> PNFSGNWKIIRSENFEELLKVLGVNVMLRKIAVAAASKPAVEIKQEGDTFYIKVSTTVRTTEINFKVGEEFEEQTVDGRPCKSLVKWE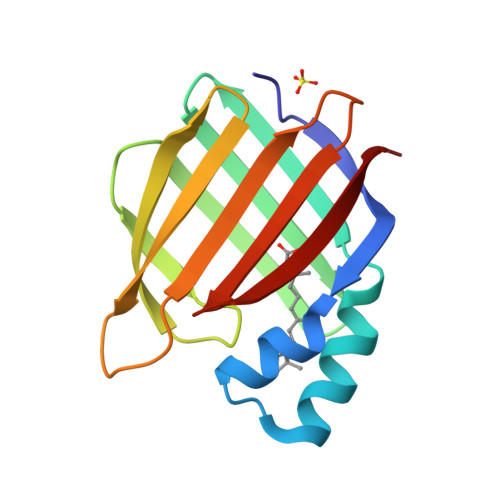SENKMVCEQKLLKGEGPKTSWTLELTNDGELIETMTADDVVCTKVFVRE> GSH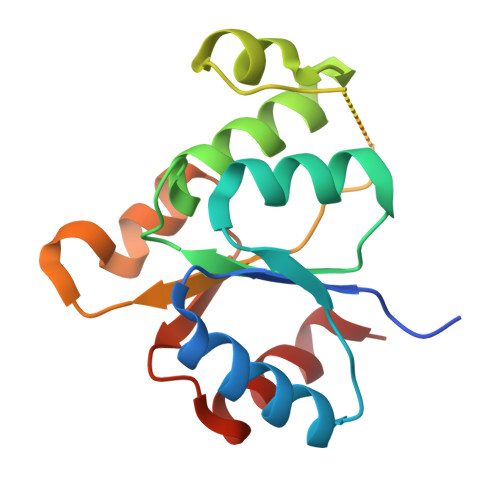METSKPKILLVEDNKINIMVAKSMMKQLGHTMDIANNGVEAITAINSSSYDLVLMDVCMPVLDGLKATRLIRSYEETGNWNAAIEAGVDISTSENEQVCMRPTNRLPIIAMTANTLAESSEECYANGMDSFISKPVTLQKLRECLQQYLH> GSSGSSGWVAFDKQVLSFDAYLEEEVLDKSQTNYRIRYYKIYFYPEDDTIQVNEPEVKNSGLLQGTSIRRHRITLPPPDEDQFYTV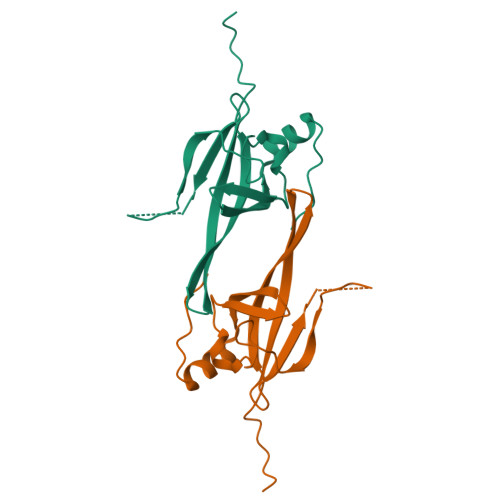YHFNVGTEVVFYGRTFKIYDCDAFTRNFLRKIGVKVNPPVQSGPSSG>[2x]MHHHHHHSSGLEVLFQGPGSDAPEEEDHVLVLRKSNFAEALAAHKYLLVEFYAPWCGHCKALAPEYAKAAGKLKAEGSEIRLAKVDATEESDLAQQYGVRGYP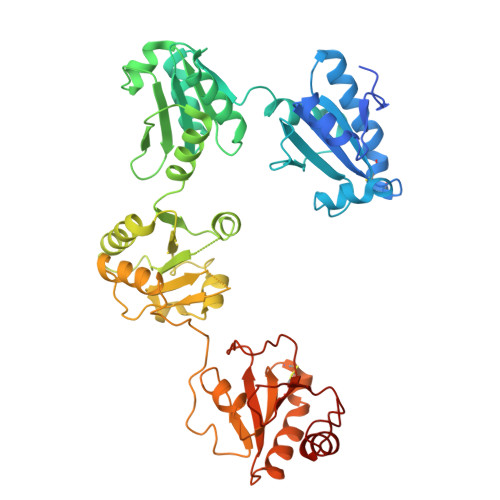TIKFFRNGDTASPKEYTAGREADDIVNWLKKRTGPAATTLPDGAAAESLVESSEVAVIGFFKDVESDSAKQFLQAAEAIDDIPFGITSNSDVFSKYQLDKDGVVLFKKFDEGRNNFEGEVTKENLLDFIKHNQLPLVIEFTEQTAPKIFGGEIKTHILLFLPKSVSDYDGKLSNFKTAAESFKGKILFIFIDSDHTDNQRILEFFGLKKEECPAVRLITLEEEMTKYKPESEELTAERITEFCHRFLEGKIKPHLMSQELPEDWDKQPVKVLVGKNFEDVAFDEKKNVFVEFYAPWCGHCKQLAPIWDKLGETYKDHENIVIAKMDSTANEVEAVKVHSFPTLKFFPASADRTVIDYNGERTLDGFKKFLESGGQDGAG> MVELTEIKDDVVQLDEPQFSRNQAIVEEKASATNNDVVDDEDDSDSDFEDEFDENETLLDRIVALKDIVPPGKRQTISNFFGFTSSFVRNAFTKSGNLAWTLTTTALLLGVPLSLSILAEQQLIEMEKTFDLQSDANNILAQGEKDAAATANGGHH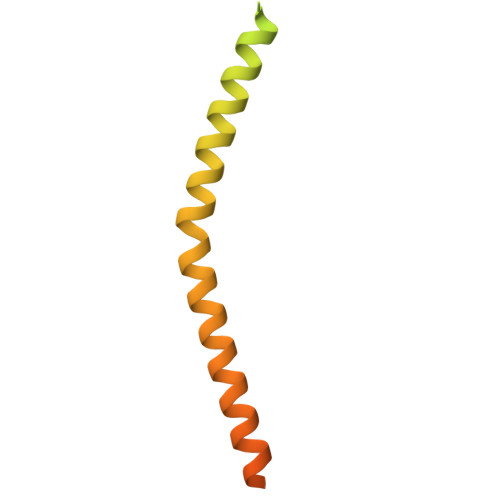HHHHHH> EKRKAEEEKRKAAAAILSLGNVLNYLDRYTVAGVLLDIQQHFGVKDRGAGLLQSVFICSFMVAAPIFGYLGDRFNRK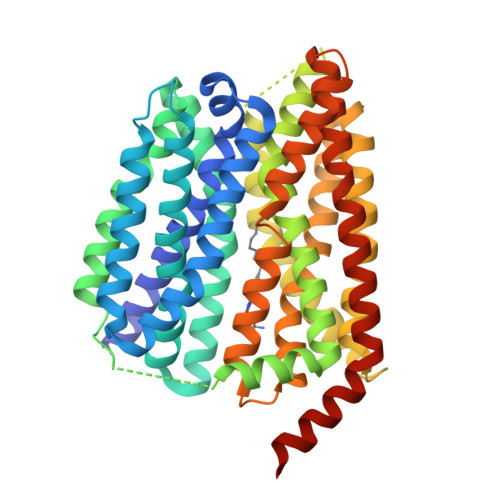VILSCGIFFWSAVTFSSSFIPQQYFWLLVLSRGLVGIGEASYSTIAPTIIGDLFTKNTRTLMLSVFYFAIPLGSGLGYITGSSVKQAAGDWHWALRVSPVLGMITGTLILILVPATKRGHADQLGDQLKARTSWLRDMKALIRNRSYVFSSLATSAVSFATGALGMWIPLYLHRAQVVQKTAETCNSPPCGAKDSLIFGAITCFTGFLGVVTGAGATRWCRLKTQRADPLVCAVGMLGSAIFICLIFVAAKSSIVGAYICIFVGETLLFSNWAITADILMYVVIPTRRATAVALQSFTSHLLGDAGSPYLIGFISDLIRQSTKDSPLWEFLSLGYALMLCPFVVVLGGMFFLATALFFVSDRARAEQQVNQLAMPPASVKV>[2x]MSMSNKLTLDKLDVKG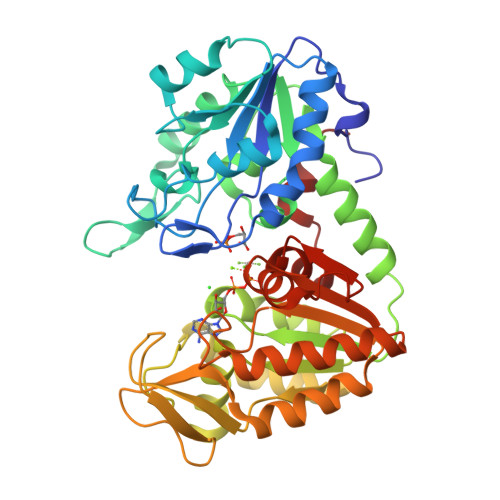KRVVMRVDFNVPMKNNQITNNQRIKAAVPSIKFCLDNGAKSVVLMSHLGRPDGVPMPDKYSLEPVAVELKSLLGKDVLFLKDCVGPEVEKACANPAAGSVILLENLRFHVEEEGKGKDASGNKVKAEPAKIEAFRASLSKLGDVYVNDAFGTAHRAHSSMVGVNLPQKAGGFLMKKELNYFAKALESPERPFLAILGGAKVADKIQLINNMLDKVNEMIIGGGMAFTFLKVLNNMEIGTSLFDEEGAKIVKDLMSKAEKNGVKITLPVDFVTADKFDENAKTGQATVASGIPAGWMGLDCGPESSKKYAEAVTRAKQIVWNGPVGVFEWEAFARGTKALMDEVVKATSRGCITIIGGGDTATCCAKWNTEDKVSHVSTGGGASLELLEGKVLPGVDALSN> RSPGTLPRKAGVFSDLSNQELKAVHSFLWSKKELRLQPSSTTTMAKNTVFLIEMLLPKKYHVLRFLDKGERHPVREARAVIFFGDQEHPNVTEFAVGPLPGPCYMRALSPRPGYQSSWASRPISTAEYALLYHTLQEATKPLHQFFLNTTGFSFQDCHDRCLAFTDVAPRGVASGQRRSWLIIQRYVEGYFLHPTGLELLVDHGSTDAGHWAVEQVWYNGKFYGSPEELARKYADGEVDVVVLEDPLPGGKGHDSTEEPPLFSSHKPRGDFPSPIHVSGPRLVQPHGPRFRLE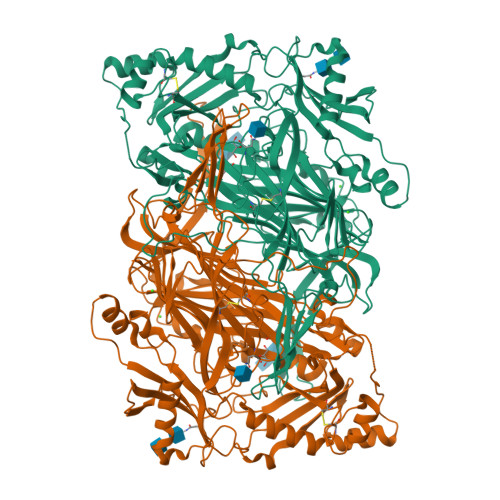GNAVLYGGWSFAFRLRSSSGLQVLNVHFGGERIAYEVSVQEAVALYGGHTPAGMQTKYLDVGWGLGSVTHELAPGIDCPETATFLDTFHYYDADDPVHYPRALCLFEMPTGVPLRRHFNSNFKGGFNFYAGLKGQVLVLRTTSTVYNYDYIWDFIFYPNGVMEAKMHATGYVHATFYTPEGLRHGTRLHTHLIGNIHTHLVHYRVDLDVAGTKNSFQTLQMKLENITNPWSPRHRVVQPTLEQTQYSWERQAAFRFKRKLPKYLLFTSPQENPWGHKRSYRLQIHSMADQVLPPGWQEEQAITWARYPLAVTKYRESELCSSSIYHQNDPWDPPVVFEQFLHNNENIENEDLVAWVTVGFLHIPHSEDIPNTATPGNSVGFLLRPFNFFPEDPSLASRDTVIVWPRDNGPNYVQRWIPEDRDCSMPPPFSYNGTYRPV> MSNIQNMSLEDIMGERFGRYSKYIIQDRALPDIRDGLKPVQRRILYSMNKDSNTFDKSYRKSAKSVGNIMGNFHPHGDSSIYDAMVRMSQNWKNREILVEMHGNNGSMDGDPPAAMRYTEARLSEIAGYLLQDIEKKTVPFAWNFDDTEKEPTVLPAAFPNLLVNGSTGISAGYATDIPPHNLAEVIDAAVYMIDHPTAKIDKLMEFLPGPDFPTGAIIQGRDEIKKAYETGKGRVVVRSKTEIEKLKGGKEQIVITEIPYEINKANLVKKIDDVRVNNKVAGIAEVRDESDRDGLRIAIELKKDANTELVLNYLFKYTDLQINYNFNMVAIDNFTPRQVGIVPILSSYIAHRREVILARSRFDKEKAEKRLHIVEGLIRVISILDEVIALIRASENKADAKENLKVSYDFTEEQAEAIVTLQLYRLTNTDVVVLQEEEAELREKIAMLAAIIGDERTMYNLMKKELREVKKKFATPRLSSLEDTAKALEHHHHHH;> MGHHHHHHHHHHSSGHIDDDDKHMSKKEININNYNDDAIQVLEGLDAVRKRPGMYIGSTDGAGLHHLVWEIVDNAVDEALSGFGDRIDVTINKDGSLTVQDHGRGMPTGMHAMGIPTVEVIFTILHAGGKFGQGGYKTSGGLHGVGSSVVNALSSWLEVEITRDGAVYKQRFENGGKPVTTLKKIGTAPKSKTGTKVTFMPDATIFSTTDFKYNTISERLNESAFLLKNVTLSLTDKRTDEAIEFHYENGVQDFVSYLNEDKEILTPVLYFEGEDNGFQVEVALQYNDGFSDNILSFVNNVRTKDGGTHETGLKSAITKVMNDYARKTGLLKEKDKNLEGSDYREGLAAVLSILVPEEHLQFEGQTKDKLGSPLARPVVDGIVADKLTFFLMENGELASNLIRKAIKARDAREAARKARDESRNGKKNKKDKGLLSGKLTPAQSKNPAKNELYLVEGDSAGGSAKQGRDRKFQAILPLRGKVINTAKAKMADILKNEEINTMIYTIGAGVGADFSIEDANYDKIIIMTDADTDGAHIQTLLLTFFYRYMRPLVEAGHVYIALPPLYKMSKGKGKKEEVAYAWTDGELEELRKQFGKGATLQRYKGLGEMNADQLWETTMNPETRTLIRVTIEDLARAERRVNVLMGDKVEPRRKWIEDNVKFTLEEATVF

Topoisomerase (topo) IV and gyrase are the type II enzymes expressed in bacteria. Topo IV mediates the unlinking of daughter chromosomes before cell division, whereas gyrase is unique in its ability to introduce negative supercoils into DNA thereby controlling chromosome supercoiling, which promotes replication fork advance and allows global regulation of gene expression. In each case, the active complex is a tetramer of two topo IV ParC and ParE subunits or gyrase GyrA and GyrB proteins. By contrast, the N-terminal and C-terminal regions of the highly conserved ParE (GyrB) subunits form the ATPase- and Mg2+-binding-TOPRIM domains, respectively.

To address this issue, we have focused on topo IV from Streptococcus pneumoniae, a Gram-positive human pathogen responsible for life-threatening infections, and for which topo IV is a target for clinically important anti-pneumococcal quinolones such as levofloxacin. Our initial attempts to crystallize a three-gate open clamp complex of S. pneumoniae topo IV used recombinant full-length ParE protein and a ParC55 protein comprising the breakage-reunion domain of ParC. A levofloxacin-DNA cleavage complex of ParE and ParC55 proteins with a 26mer E-site DNA yielded a crystal structure in the rhombohedral space group H32 with a best resolution of 6.5 Å. One complex involving E-site DNA stabilized with levofloxacin was solved at 6.5 Å; a second structure containing V-site DNA and no drug was solved at 3.7 Å resolution, revealing two different DNA-binding sites. Essentially, the same open clamp conformation and domain dispositions were seen for this drug-free complex as was observed for the levofloxacin-stabilized 6.5 Å complex obtained in a different space group using a different gate-DNA sequence and different crystallization conditions. However, the absence of ATPase domains leads to some uncertainties in modelling the scope and accessibility of drug binding pockets, as suggested by the closed clamp structure in which the ATPase domains adopt the criss-cross conformation and partially shield the DNA binding groove from the solvent above. Reassuringly, the open clamp structure of full-length topo IV reveals that the ATPase domains are folded back, and the DNA gate is fully accessible to drugs from solvent above (Figure 10B and in the lower resolution levofloxacin complex, Supplementary Section).> MLRNHKLSKVFSATAISLFLSSTAFADTTVRMMHIETDPNVLGVWEEIAKDFEAKNPDIKVNLEFLENEAFKAKLPTLLQSQQKPDLFYSWGGGNFQVRAESGLLEDMEGYSATLNQELSAAGMNAFKIDGKQYGAPYMVSQVGFWYNKKLFKQAGIDGESIQTWDEFLTAIEKLKAAGITPIAVGGADKWPMHFYWSYLAMRAGGQEAFAAAMQDQGDGFAGEAFVRAGEELKRLAALEPFQPGFMAAGYGESAGLFGDYKAAIHLMGDWDYNFQAQQAVDKKGVVDSDLGFMNFPVLKGGAGAGSDTLGGINGFAFAKGAKPEA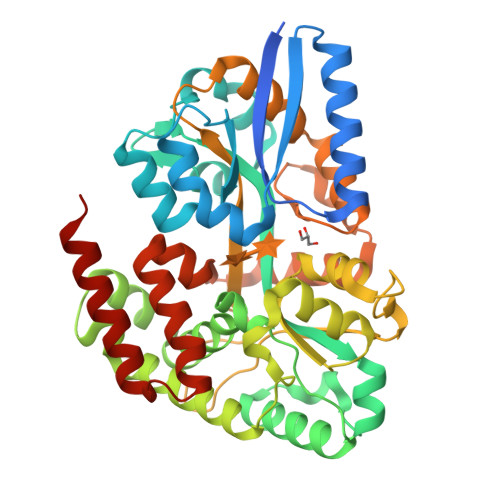AKWLEFFLNENSQTKLAEIDQIIPVAKGADKGLKNPFKQKISQTISSAQWHQVFFDQALGADVGGVVNDISVGIVNGDVTPKEAAEQVQEAWEMRLEHHHHHH> GSHKIRVGDALLGRLIDGIGRPMESNIVAPYLPFERSLYAEPPDPLLRQVIDQPFI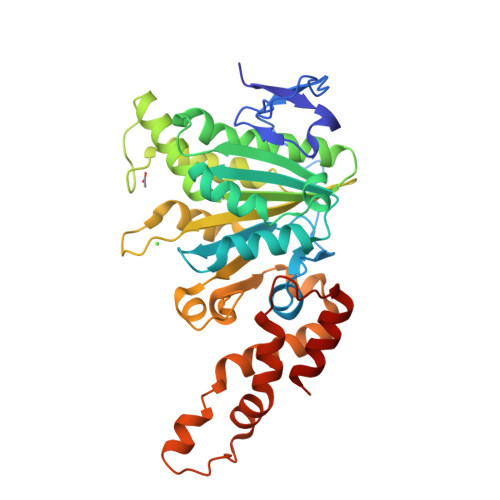LGVRAIDGLLTCGIGQRIGIFAGSGVGKSTLLGMICNGASADIIVLALIGERGREVNEFLALLPQSTLSKCVLVVTTSDRPALERMKAAFTATTIAEYFRDQGKNVLLMMDSVTRYARAARDVGLASGEPDVRGGFPPSVFSSLPKLLERAGPAPKGSITAIYTVLLESDNVNDPIGDEVRSILDGHIVLTRELAEENHFPAIDIGLSASRVMHNVVTSEHLRAAAECKKLIATYKNPELLIRIGEYTMGQDPEADKAIKNRKLIQNFIQQSTKDISSYEKTIESLFKVVA>MGSSHHHH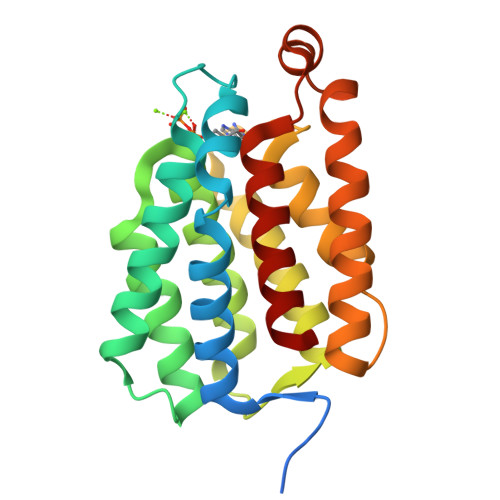HHSSGENLYFQGHMAEAWGPEAVAEAFRYATRWFQVYVEELNALNVYPVPDGDTGTNMLHTLEAARRELDLADTSRMDQVARALAYGSLLGARGNSGVILSQILRGFAEALKGKRALDGSLLRRALRMGAESGYKAVMRPVEGTILTVARAAGEGARGEALEEVLETALEAAREALERTPELLPVLRQAGVVDAGGAGYVRLLEGMRGYAL[2x]> ETPPRFTRTPVDQTGVSGGVASFICQATGDPRPKIVWNKKGKKVSNQRFEVIEFDDGSGSVLRIQPLRTPRDEAIYECVASNNVGEISVSTRLTVLREDQIPRGFPTIDMGPQLKVVERTRTATMLCAASGNPDPEITWFKDFLPVDTSNNNGRIKQLRSESIGGTPIRGALQIEQSEESDQGKYECVATNSAGTRYSAPANLYVRELREVRRVPPRFSIPPTNHEIMPGGSVNITCVAVGSPMPYVKWMLGAEDLTPEDDMPIGRNVLELNDVRQSANYTCVAMSTLGVIEAIAQITVKALPKPPGTPVVTESTATSITLTWDSGNPEPVSYYIIQHKPKNSEEPYKEIDGIATTRYSVAGLSPYSDY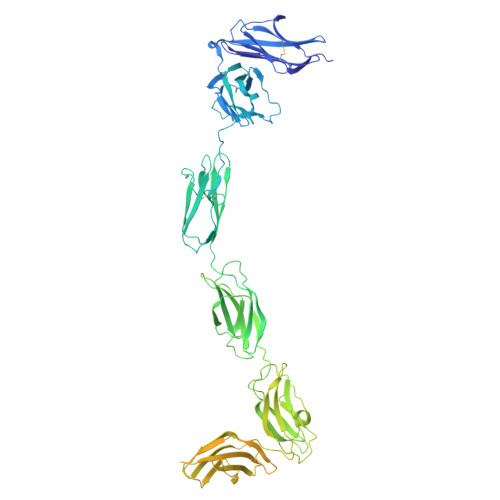EFRVVAVNNIGRGPASEPVLTQTSEQAPSSAPRDVQARMLSSTTILVQWKEPEEPNGQIQGYRVYYTMDPTQHVNNWMKHNVADSQITTIGNLVPQKTYSVKVLAFTSIGDGPLSSDIQVITQTGVPGQPLNFKAEPESETSILLSWTPPRSDTIASYELVYRDGDQGEEQRITIEPGTSYRLQGLKPNSLYYFRLSARSPQGLGASTAEISARTMQSMFAKNFHVKAVMKTSVLLSWEIPENYNSAMPFKILYDDGKMVEEVDGRATQKLIVNLKPEKSYSFVLTNRGNSAGGLQHRVTAKTAPDVLRTKPAFIGKTNLDGMITVQLPDVPANENIKGYYIIIVPLKKSRGKFIKPWESPDEMELDELLKEISRKRRSIRYGREVELKPYIAAHFDVLPTEFTLGDDKHYGGFTNKQLQSGQEYVFFVLAVMDHAESKMYATSPYSDPVVSMDLDPQPITDEEEKHHHHHH>MAHHHHHHVDDDDKMAPAYLTTHNRTGEESNAYIAGSIPSLYPTAAYSTNQVYWNLVRLACYGHTTNGQCPALIKMATNTANPIDIGYVTMDLNTGDITPKTLSAKGYSLRVIGPGEAEITKN[2x]

L. pneumophila also expresses a type II secretion system (T2SS). The Legionella T2SS exports at least 25 proteins. In summary, using a combined cellular, structural, biophysical and biochemical approach we have provided a characterization of three novel type II secreted substrates, NttA, NttC and NttE, that are required for infection of several species of amoeba. We also report the X-ray crystal structures of NttE and NttC, the solution nuclear magnetic resonance (NMR) structure of NttA and dynamic analyses for each substrate using complementary biophysical techniques.

NttC is a 130-amino acid protein encoded by the lpw18401 ORF in 130b strain (lpg1809 in strain Philadelphia-1; lpp1772 in strain Paris; lpl1773 in strain Lens). We readily obtained crystals of NttC at pH 8.0 and determined its structure using selenium multi-wavelength anomalous dispersion (Se-MAD) and refined electron density maps to 3.1 Å. The final model of NttC contains two identical molecules in the asymmetric unit (RMSD over Cα atoms of 0.080 Å) and all residues could be built except for the N-terminal His6 tags. NttC has an immunoglobulin-like fold composed of one α-helix and ten β-strands, and residues Cys46 and Cys55 form a disulfide bond between the α1-helix and β5-strand. However, NttC is unusual in that it lacks a compact core and instead contains a buried internal cavity. This is formed primarily by the sidechains of hydrophobic residues and is inaccessible to the solvent. Analysis of the structure using fpocket revealed that the cavity inside the protein has a volume of 782 Å3 and a druggability score of 0.97, which strongly suggests that this pocket may be able to bind one or more organic molecules. Furthermore, when we analyzed all known sequences of NttC homologs and mapped the sequence conservation onto the NttC structure, we observed only minor patches on the NttC surface while many of the residues that form the internal cavity were highly conserved. In our crystal structure, we could not detect any access to the cavity but using MD we were able to observe a breathable core and a transient ∼12 Å diameter solvent accessible channel form over the course of the simulations. Due to the restricted access to this pocket we expect that a large cofactor is inserted during the folding of NttC, prior to its secretion from the periplasm.>QLTPTFYRETCPNLFPIVFGVIFDASFTDPRIGASLMRLHFHDCFVQGCDGSVLLNNTDTIESEQDALPNINS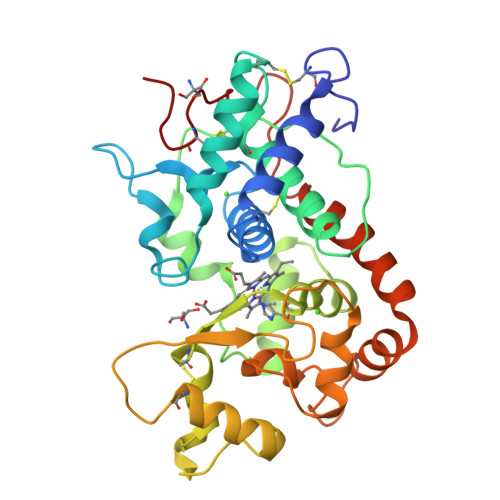IRGLDVVNDIKTAVENSCPDTVSCADILAIAAEIASVLGGGPGWPVPLGRRDSLTANRTLANQNLPAPFFNLTQLKASFAVQGLNTLDLVTLSGGHTFGRARCSTFINRLYNFSNTGNPDPTLNTTYLEVLRARCPQNATGDNLTNLDLSTPDQFDNRYYSNLLQLNGLLQSDQELFSTPGADTIPIVNSFSSNQNTFFSNFRVSMIKMGNIGVLTGDEGEIRLQCNFVNG[3x]>[60x]MNNLYRDLAPVTEAAWAEIELEAARTFKRHIAGRRVVDVSDPGGPVTAAVSTGRLIDVKAPTNGVIAHLRASKPLVRLRVPFTLSRNEIDDVERGSK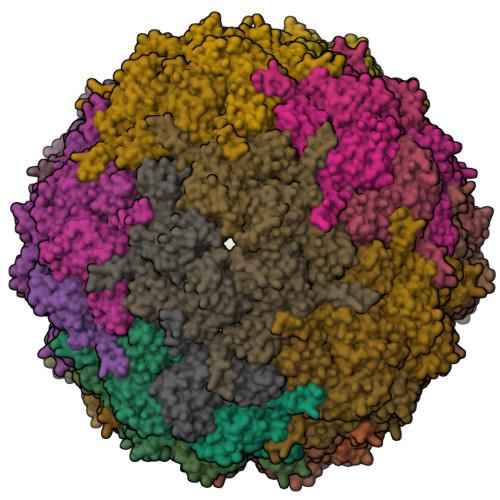DSDWEPVKEAAKKLAFVEDRTIFEGYSAASIEGIRSASSNPALTLPEDPREIPDVISQALSELRLAGVDGPYSVLLSADVYTKVSETSDHGYPIREHLNRLVDGDIIWAPAIDGAFVLTTRGGDFDLQLGTDVAIGYASHDTDTVRLYLQETLTFLCYTAEASVALSHHHHHH> SPMGVLLRMIPAVGHFIPITSITLIYYRLYLEDITFHLYLVPNDCTIRKAIDEEELKFQFVRINKPPPVDALYVGSRYIVSSSKEVEILPKE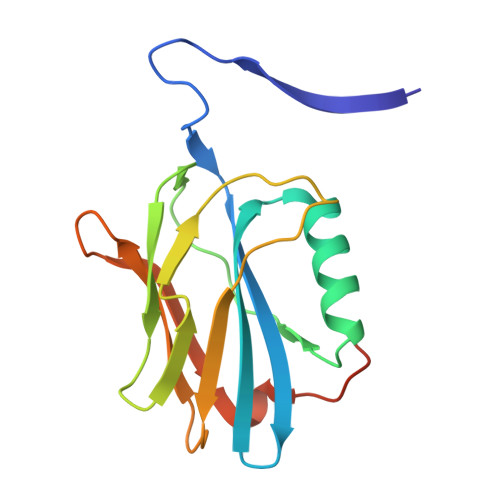LELCYRSPRESQLFSEIYVGNIGSGINLQLTDKKYMNLIWEALLKPGDLRPALPRMASAPKD>[2x]SELDAKLNKLGVDRIAISPYKQWTRGYMEPGNIGNGYVTGLKVDAGVRDKSDDDVLDGIVSYDRAETKNAYIGQINMTTAS;>XFTGVQGRVIGYDIL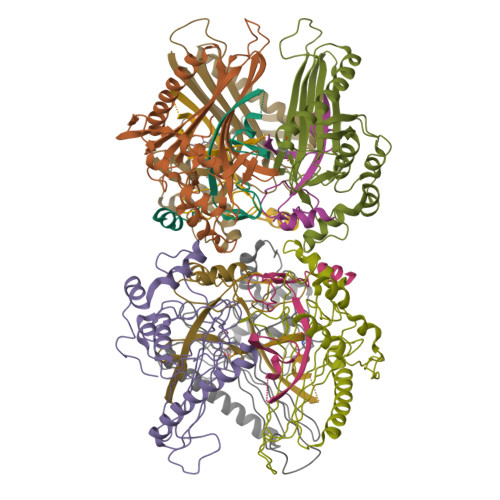RSPEVDKAKPLFTETQWDGSELPIYDAKPLQDALVEYFGTEQDRRHYPAPGSFIVCANKGVTAERPKNDADMKPGQGYGVWSAIAISFAKDPTKDSSMFVEDAGVWETPNEDELLEYLEGRRKAMAKSIAECGQDAHASFESSWIGFAYTMMEPGQIGNAITVAPYVSLPIDSIPGGSILTPDKDMEIMENLTMPEWLEKMGYKSLSANNALKY[2x]> HPETLVKVKDAEDQLGARVGYIELDLNSGKILESFRPEERFPMMSTFKVLLCGAVLSRVDAGQEQLGRRIHYSQNDLVEYSPVTEKHLTDGMTVRELCSAAITMSDNTAANLLLTTIGGPKELTAFLHNMGDHVTRLDRYYGELNEAIPN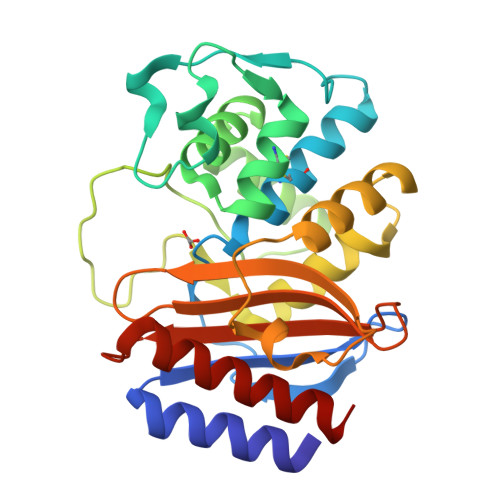DERDTTMPAAMATTLRKLLTGELLTPASRQQLIDWMEADKVAGPLLRSALPAGWFIADKSGAGERGSRGIIAALGPDGKPSRIVVIYTTGSQATMDERNRQIAEIGASLIKHW> MAKPANKLVIVTEKILLKKIAKIIDESGAKGYTVMNTGGKGSRNVRSSGQPNTSDIEANIKFEILTETREMAEEIADRVAVKYFNDYAGIIYICSAEVLY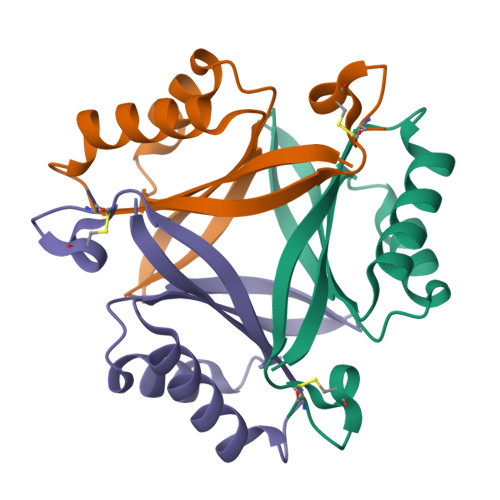GHTFCGPEGCSAWSHPQFEK>[4x]MNHKVHHHHHHMELQDVVVKGPDEKLQLAVFVQNETKPCYSVSYNGKTMLEKSPLGMNTNIG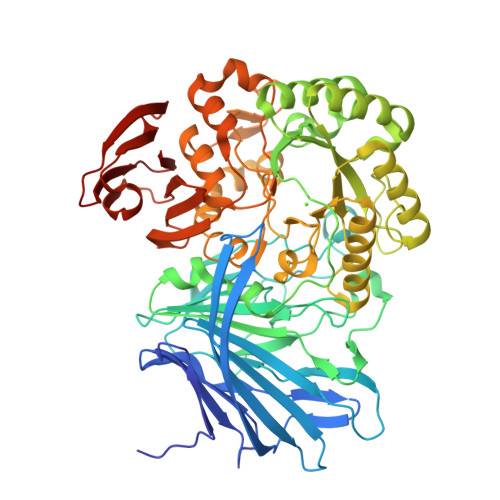DFTKNLKLTGHSVDKIDTVYQQTRIKVSNVHYRANELTCHLENEQGQKLGVIFRVSDNDVAFRYTLPHQGGKASVTVKEEQTGFRFPEQTTTFLCPQSDAMIGWKRTKPSYEEEYKADAPMSDRSQYGHGYTFPCLFRIGNDGWVLVSETGVDSRYCGSRLSDVSEGNLYTVAFPMAEENNGNGTVAPAFALPGATPWRTITVGDHLKPIVETTVPWDVVSPLYETKHDYRFGRGTWSWILWQDGSINYDDQVRYIDFASAMGYEYALIDNWWDTRIGHQRMKSLVEYARDKGVELFLWYSSSGYWNDIEQGPVNRMDNAIIRKREMKWLQSLGVKGIKVDFFGGDKQETMRLYEDILSDADDHGLMVIFHGCTLPRGWERMYPNYVGSEAVLASENMVFNQHFCDEEAFNTCLHPFIRNTVGSMEFGGCLLNKRLNRNNDGGTTRRTTDVFQLATTVLLQNPVQNFALAPNNLKDVPAVCMDFMKRVPTTWDETRFVDGYPGKYVVLARRQGDTWYLAAVNAGKEPLKLKLDLEMFAGKTVALYKDDKKGEPELTSLKVKENGKVQLEIRPQGGILCIK> RGH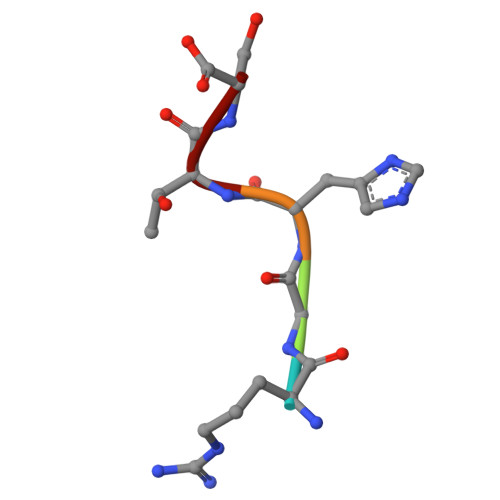TS>MDIKINDITLGNNSPFVLFGGINVLESLDSTLQTCAHYVEVTRKLGIPYIFKASFDKANRSSIHSYRGVGLEEGLKIFEKVKAEFGIPVITDVHEPHQCQPVAEVCDVIQLPAFLARQTDLVVAMAKTGNVVNIKKPQFLSPSQMKNIVEKFHEAGNGKLILCERGSSFGYDNLVVDMLGFGVMKQTCGNLPVIFDVTHSLATRDAGSAASGGRRAQALDLALAGMATRLAG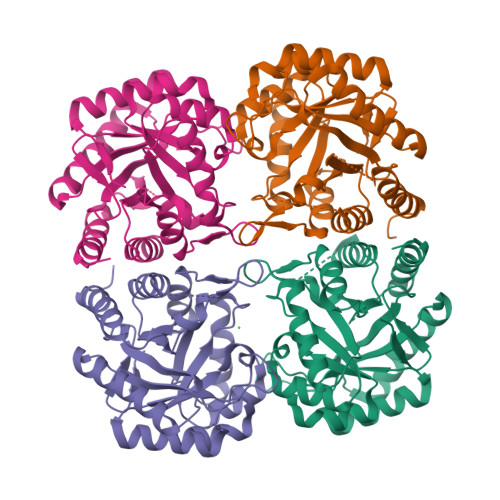LFLESHPDPKLAKCDGPSALPLHLLEDFLIRIKALDDLIKSQPILTIE[4x]>[4x]MSFNANLDTLYRQVIMDHYKNPRNKGVLNDSIVVDMNNPTCGDRIRLTMKLDGDIVEDAKFEGEGCSISMASASMMTQAIKGKDIETALSMSKIF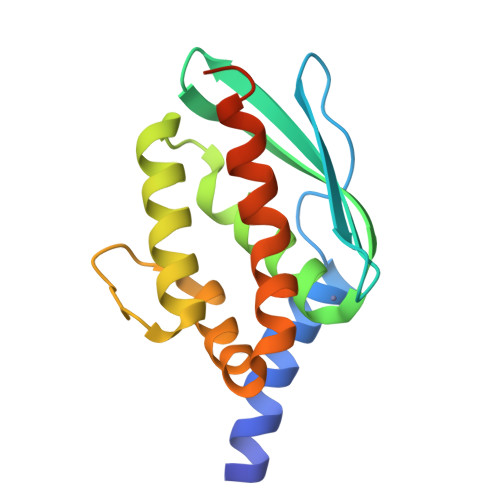SDMMQGKEYDDSIDLGDIEALQGVSKFPARIKCATLSWKALEKGVAKEEGGNLEHHHHHH> QDQEKGITIDISRKHYTVETLKSLVDEISYNGGNYVQLHFSDNENYAIASEYLGQSSENTNNTYLTKNELLSLIAYSNDKDILVIPDIDLPAHSKGWLELIKKKDVKLYNDIVTDYSEETLDYYDNRVALDTVNQLLDEVLDLFYQPKFEGKQRIVLGGDEVSGSEVHQLDFIDFMNQIASTVKESKYEPQMWNDSITSEGIANLDDSFSILYWQQS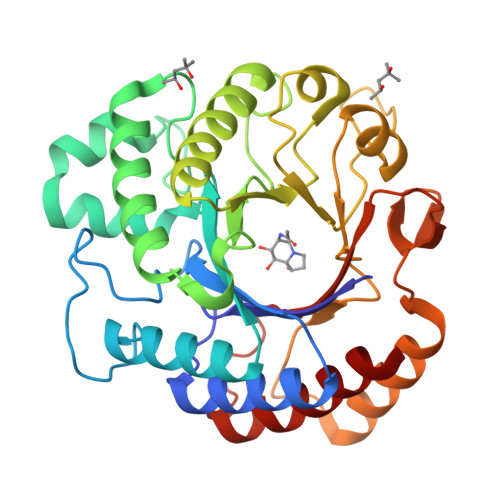TLSSGEESLNVEDFENWGFSVYNYNAYSLYFLPSNGFTQEDINEQMDYMNWAYAHNKFFYISDYYHAVETSNVKGSSLTFWGEHATDLSQKKLLKQELPLIRHYLNL> MKLMAQLGKLLKEQKYDRQLRLWGDHGQEALESAHVCLINATATGTEILKNLVLPGIGSFTIIDGNQVSGEDAGNNFFLQRSSIGKNRAEAAM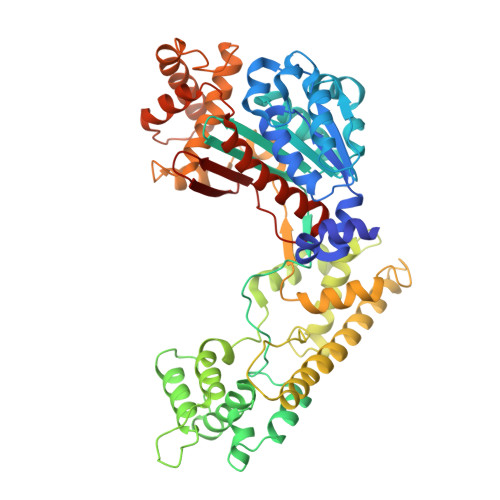EFLQELNSDVSGSFVEESPENLLDNDPSFFCRFTVVVATQLPESTSLRLADVLWNSQIPLLICRTYGLVGYMRIIIKEHPVIESHPDNALEDLRLDKPFPELREHFQSYDLDHMEKKDHSHTPWIVIIAKYLAQWYSETNGRIPKTYKEKEDFRDLIRQGILKNENGAPEDEENFEEAIKNVNTALNTTQIPSSIEDIFNDDRCINITKQTPSFWILARALKEFVAKEGQGNLPVRGTIPDMIADSGKYIKLQNVYREKAKKDAAAVGNHVAKLLQSIGQAPESISEKELKLLCSNSAFLRVVRCRSLAEEYGLDTINKDEIISSMDNPDNEIVLYLMLRAVDRFHKQQGRYPGVSNYQVEEDIGKLKSCLTGFLQEYGLSVMVKDDYVHEFCRYGAAEPHTIAAFLGGAAAQEVIKIITKQFVIFNNTYIYSGMSQTSATFQL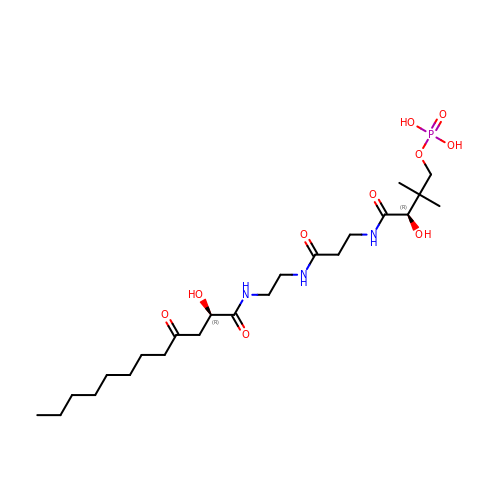N~3~-[(2R)-2-hydroxy-3,3-dimethyl-4-(phosphonooxy)butanoyl]-N-{2-[(2R)-2-hydroxy-4-oxododecanamido]ethyl}-beta-alaninamide | C23 H44 N3 O10 P | BTRNTPSBBUMIHA-QUCCMNQESA-N>MRAEGLGGLERFCSPGKGRGLRALQPFQVGDLLFSCPAYAYVLTVNERGNHCEYCFTRKEGLSKCGRCKQAFYCNVECQKEDWPMHKLECSPMVVFGENWNPSETVRLTARILAKQKIHPERTPSEKLLAVKEFESHLDKLDNEKKDLIQSDIAALHHFYSKHLGFPDNDSLVVLFAQVNCNGFTIEDEELSHLGSAIFPDVALMNHSCCPNVIVTYKGTLAEVRAVQEIKPG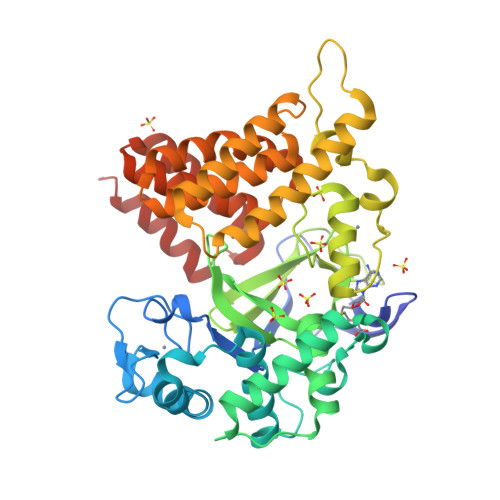EEVFTSYIDLLYPTEDRNDRLRDSYFFTCECQECTTKDKDKAKVEIRKLSDPPKAEAIRDMVRYARNVIEEFRRAKHYKSPSELLEICELSQEKMSSVFEDSNVYMLHMMYQAMGVCLYMQDWEGALQYGQKIIKPYSKHYPLYSLNVASMWLKLGRLYMGLEHKAAGEKALKKAIAIMEVAHGKDHPYISEIKQEIESHLEHHHHHH[2x]2-(butylamino)-N-[(2S,3S,5R)-6-(butylamino)-3-hydroxy-5-methyl-6-oxo-1-phenylhexan-2-yl]-6-methoxypyridine-4-carboxamide 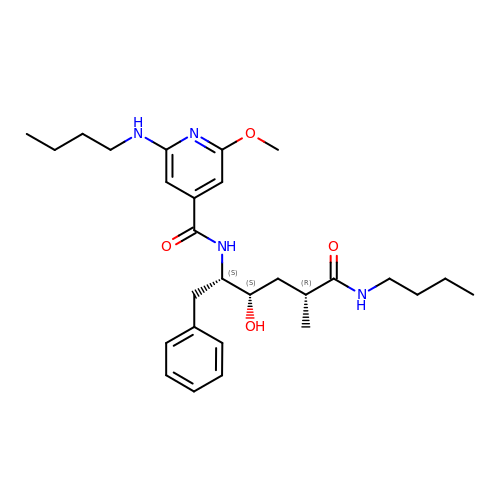| C28 H42 N4 O4 | XXAQWIHKXZOYLW-QDSKXPNFSA-N> KIPNFVVPGKCASVDRNKLWAEQTPNRNSYAGVWYQFALTNNPYQLIEKCVRNEYSFDGKQFVIKSTGIAYDGNLLKRNGKLYPNPFGEPHLSIDYENSFAAPLVILETDYSNYACLYSCIDYNFGYHSDFSFIFSRSANLADQYVKKCEAAFKNINVDTTRFVKTVQGSSCPYDTQKTV;> DGIPSFVTAGKCASVANQDNFDLRRYAGRWYQTHIIENAYQPVTRCIHSNYEYSTNDYGFKVTTAGFNPNDEYLKIDFKVYPTKEFPAAHM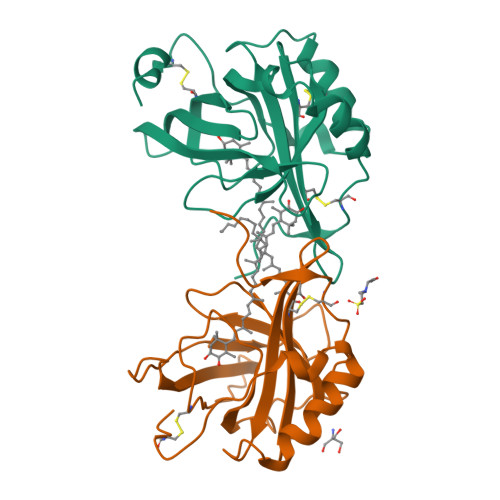LIDAPSVFAAPYEVIETDYETYSCVYSCITTDNYKSEFAFVFSRTPQTSGPAVEKTAAVFNKNGVEFSKFVPVSHTAECVYRA>MSVIKSDMKIKLRMEGTVNGHKFVIEGEGEGKPYEGTQTMNLKVKEGAPLPFAYDILTTAFQYGNRVFTKYPKDIPDYFKQSFPEGYSWERSMTFEDGGICTATSDITLEGDCFFYEIRFDGVNFPPNGPVMQKKTLKWEPSTEKMYVRDGVLMGDVNMALLLEGGGHYRCDFKTTYKAKKGVQLPDYHFVDHRI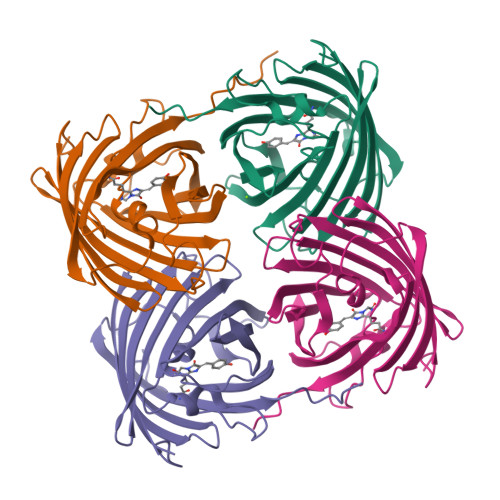EILSHDKDYNNVKLYEHAVARSSLLPMTAAHHHHHH[4x]>DDSCQIGTSFTGLDMTKYVGTWYELFRTPNSDEEDFTNCEYDKYTLDENGVIQVTSVAYTNSIRGFITSTGTVPSWTEDTFDIAYGDDETWSSTYFMVGTDYQTYSIVAGCLDNDYSRHLYWIASHETSFDDA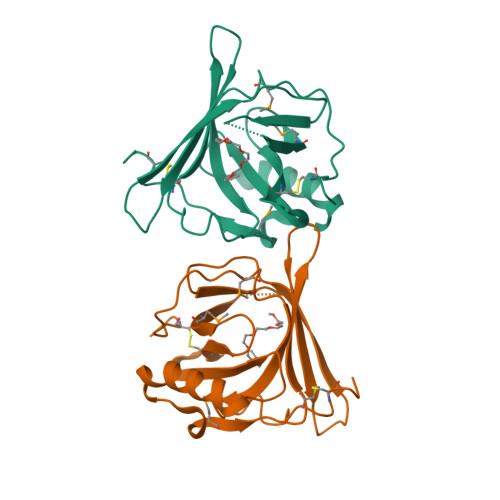TKAKVNEVLAPYNLSLDDMEPVDQSYCVQY[2x]>[2x]STAGKVIKCKAAVLWEEKKPFSIEEVEVAPPKAHEVRIKMVATGICRSDDHVVSGTLVTPLPVIAGHEAAGIVESIGEGVTTVRPGDKVIPLFTPQCGKCRVCKHPEGNFCLKNDLSMPRGTMQDGTSRFTCRGKPIHHFLGTSTFSQYTVVDEISVAKIDAASPLEKVCLIGCGFSTGYGSAVKVAKVTQGSTCAVFGLGGVGLSVIMGCKAAGAA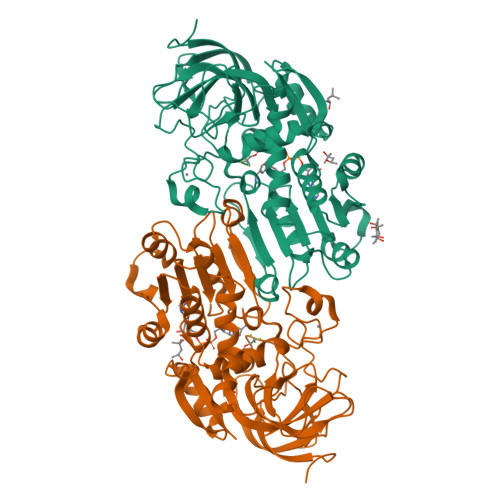RIIGVDINKDKFAKAKEVGATECVNPQDYKKPIQEVLTEMSNGGVDFSFEVIGRLDTMVTALSCCQEAYGVSVIVGVPPDSQNLSMNPMLLLSGRTWKGAIFGGFKSKDSVPKLVADFMAKKFALDPLITHVLPFEKINEGFDLLRSGESIRTILTF> MAASQEIFLQVLNLADGDVKVTVLGSRNNSLLVESVSSFQNTTHYSKLHLEAKSQDLHFHLKYNSLSVHNDHSVEEKNCYQLLIHQDGESISSMLVKDTGIKPANGMAAIRFINTLHKDLNISLDTDAPLSVGKDYGVSAYRTVLRGKYPAVHCETEDKVFSLDLGQLDF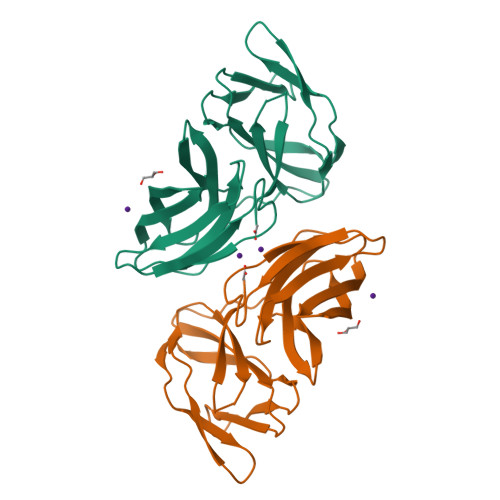GTTYLFVITNITSQGLQAWKAEDI>MAKIDNAVLPEGSLVLVTGANGFVASHVVEQLLEHGYKVRGTARSASKLANLQKRWDAKYPGRFETAVVEDMLKQGAYDEVIKGAAGVAHIASVVSFSNKYDEVVTPAIGGTLNALRAAAATPSVKRFVLTSSTVSALIPKPNVEGIYLDEKSWNLESIDKAKTLPESDPQKSLWVYAASKTEAELAAWKFMDENKPHFTLNAVLPNYTIGTIFDPETQSGSTSGWMMSLFNGEVSPALALFPPTYYVSAVDIGLLHLGCLVLPQIERRRVYGTAGTFDWNTVLATFRKLYPSKTFPADFPDQGQDLSKFDTAPSLEILKSLGR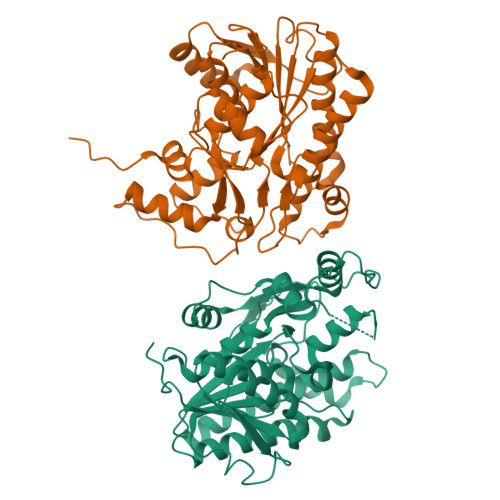PGWRSIEESIKDLVGSETAIQ[2x]>MDLYAVWGNPIAQSKSPLIQNKLAAQTHQTMEYIAKLGDLDAFEQQLLAFFEEGAKGCNITSPFKERAYQLADEYSQRAKLAEACNTLKKLDDGKLYADNTDGIGLVTDLQRLNWLRPNQHVLILGAGGATKGVLLPLLQAQQNIVL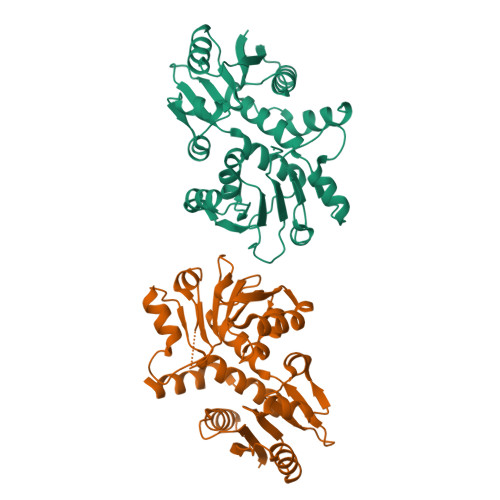ANRTFSKTKELAERFQPYGNIQAVSMDSIPLQTYDLVINATSAGLSGGTASVDAEILKLGSAFYDMQYAKGTDTPFIALCKSLGLTNVSDGFGMLVAQAAHSFHLWRGVMPDFVSVYEQLKKAML[2x]>GAMDPSSPNYDKWEMERTDITMKHKLGGGQYGEVYEGVWKKYSLTVAVKTLKEDTMEVEEFLKEAAVMKEIKHPNLVQLLGVCTREPPFYIITEFMTYGNLLDYLRECNRQEVSAVVLLYMATQISSAMEYLEKKNFIHRDLAARNCLVGENHLVKVADFGLSRLMTGDTYTAHAGAKFPIKWTAPESLAYNKFSIKSDVWAFGVLLWEIATYGMSPYPGIDLSQVYELLEKDYRMERPEGCPEKVYELMRACWQWNPSDRPSFAEIHQAFETMFQESSISDEVEKELG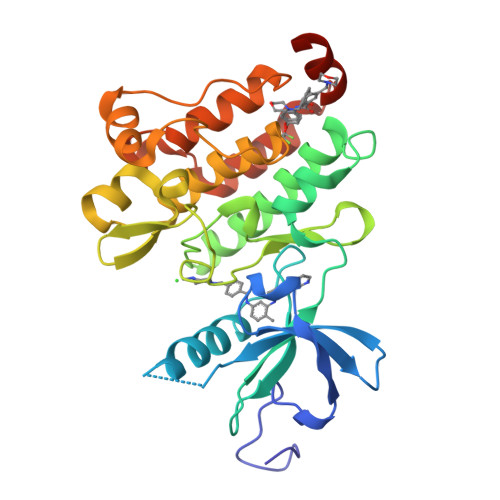KRGT[2x]>[2x]SNAMVDFRKFYKENANVAYTVLGYPNLQTSEAFLQRLDQSPIDILELGVAYSDPIADGEIIADAAKIALDQGVDIHSVFELLARIKTKKALVFMVYYNLIFSYGLEKFVKKAKSLGICALIVPELSFEESDDLIKECERYNIALITLVSVTTPKERVKKLVKHA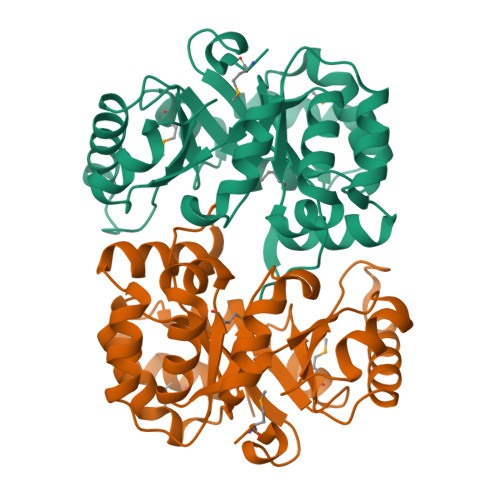KGFIYLLASIGITGTKSVEEAILQDKVKEIRSFTNLPIFVGFGIQNNQDVKRMRKVADGVIVGTSIVKCFKQGNLDIIMKDIEEIFKK> PLTEIQVESYKKALQADVPPEKRENVGIQAAFKETFPIEEGDKGKGGLVLDFLEYRIGDPPFSQDECREKDLTYQAPLYARLQLIHKDTGLIKEDEVFLGHLPLMTEDGSFIINGADRVIVSQGGRTVGELMADQFRVGLARLARGVRERMVM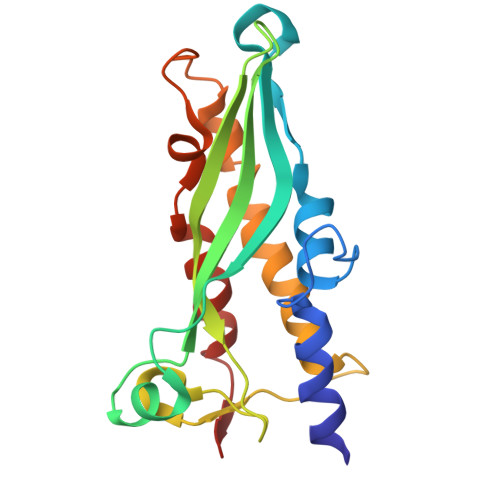GSPDTLTPAKLVNSRPLEAALREFFSRSQLS>[3x]AKCVSYGVSQIKAPALHSQGYTGSNVKVAVIDSGIDSSHPDLNVAGGASFVPSETNPFQDNNSHGTHVAGTVLAVAPSASLYAVKVLGADGSGQYSWIINGIEWAIANNMDVINMSLGGPSGSAALKAAVDKAVASGVVVVAAAGNSGTSGSSSTVSYPAKYPSVIAVGAVDSSNQRAPWSSVGPELDVMAPGVSICSTLPGNKYGAHSGTCPASNHVAGAAALILSKHPNWTNTQVRSSLENTATKLGDSFYYGKGLINVEAAAQHHHHHH;> LPEGSPVTLDLRY

Omniligase-1 is a broadly applicable enzyme for peptide bond formation between an activated acyl donor peptide and a non-protected acyl acceptor peptide. The enzyme is derived from an earlier subtilisin variant called peptiligase by several rounds of protein engineering aimed at increasing synthetic yields and substrate range. Mutation A225N in the S1′ pocket and F189W of the S2′ pocket increased the synthesis to hydrolysis (S/H) ratio and overall coupling efficiency, whereas the I107V mutation was added to S4 pocket to increase the reaction rate. The final omniligase variants appeared to have a very broad substrate range, coupling more than 250 peptides in a 400-member library of acyl acceptors, as indicated by a high-throughput FRET assay.

Thus, Oml-1 and other omniligase variants containing mutation F189W, which is crucial for the broad substrate scope, cannot be crystallized in crystal form A or B. Crystals of variants containing a Trp at position 189 were only found after a long incubation time for Pre-4 (Ptl-M222P/L217H/A225N/F189W) and Pre-5 (Ptl-M222P/L217H/A225N/F189W/N218D). The structures of Pre-4 and Pre-5 each contain three protein molecules in the asymmetric unit (molecules A-C). In both of these variants Trp189 is involved in intermolecular contacts which are different from those in Pre-1-Pre-3. In addition to the role of Phe189 in crystal formation, we observed that for both Pre-4 and Pre-5, crystallization resulted in at least one substrate binding site occupied by a peptide sequence. Variants Pre-4 and Pre-5 crystallized in crystal form C containing three protein molecules (A, B and C) in the asymmetric unit. In crystal form C the structure of molecule C is more different with RMSDs of 0.6 – 0.7 Å to molecules A and B. It has an oxidized cysteine and a bound eglin fragment (41′-46′ (SPVTLAG P5 -P1′)) that was used as a crystallization aid. In this crystal form C, we also observed a crystallization artifact; part of the loop from Ile205 to His217 of molecule C is forcibly drawn into the active site of molecule B, mimicking a peptide substrate. Hence, the conformation of the five N-terminal residues of chain C (AKCVG) also changed. This is an example of a crystallization artifact, and shows that ligases have a strong preference for binding a peptide in the active site even if it is their sibling. The second effect is due to F189W in the S2′ pocket, which serves as a strong binding force to drive the binding of substrates with hydrophobic residues at P2′.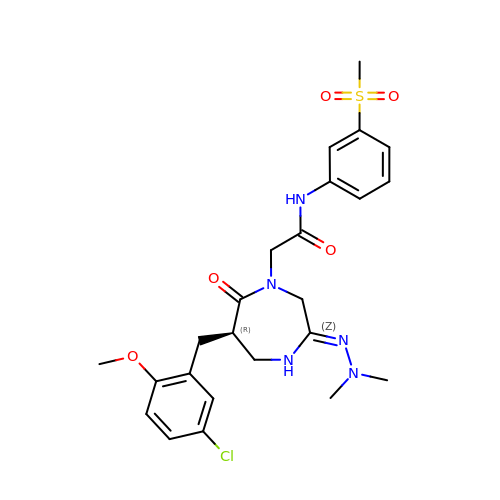(R)-2-(6-(5-chloro-2-methoxybenzyl)-3-(2,2-dimethylhydrazono)-7-oxo-1,4-diazepan-1-yl)-N-(3-(methylsulfonyl)phenyl)acetamide | C24 H30 Cl N5 O5 S | NWZUZBYLXNQLIF-QGZVFWFLSA-N>KPGAPWWKSAVFYQVYPRSFKDTNGDGIGDFKGLTEKLDYLKGLGIDAIWINPHYASPNTDNGYDISDYREVMKEYGTMEDFDRLMAELKKRGMRLMVDVVINHSSDQHEWFKSSRASKDNPYRDYYFWRDGKDGHEPNNYPSFFGGSAW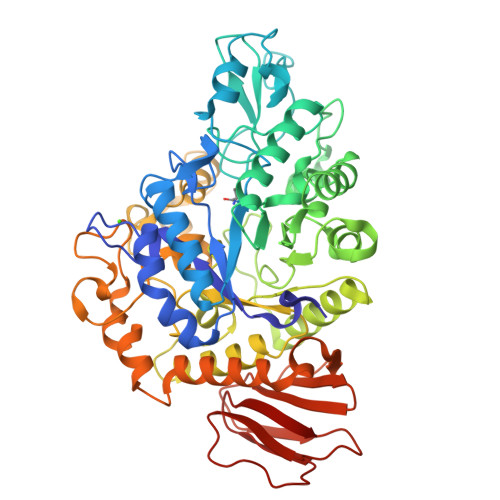EKDPVTGQYYLHYFGRQQPDLNWDTPKLREELYAMLRFWLDKGVSGMRFDTVATYSKTPGFPDLTPEQMKNFAEAYTQGPNLHRYLQEMHEKVFDHYDAVTAGEIFGVPLNQVPLFIDSRRKELDMAFTFDLIRYDRALDRWHTIPRTLADFRQTIDKVDAIAGEYGWNTFFLGNHDNPRAVSHFGDDRPQWREASAKALATVTLTQRGTPFIFQGDELGMTNYPFKTLQDFDDIEVKGFFQDYVETGKATAEELLTNVALTSRDNARTPFQWDDSANAGFTTGKPWLKVNPNYTEINAAREIGDPKSVYSFYRNLISIRHETPALSTGSYRDIDPSNADVYAYTRSQDGETYLVVVNFKAEPRSFTLPDGMHIAETLIESSSPAAPAAGAASLELQPWQSGIYKVK[2x]> MPQLHYVPYDTPVEDVMRILKESGTLVIRNFLDQNTVQKVQDEVDDYVRNWNPGPGSKTKQPSNLSLMSKTYRCEVLNHPWMHAICERMFGPTYGDYWFNGGSILHLEPGENTQPIHQDHVFYQISKWRRPTDPDLTINFTMALTEFTVENGGTRVCPGSHLWENGHASPAEEDMVPVLMQPGDALILPGSMWHSAGANRTSEYRRGFATSFHPCHFTPIESHHHLPREMVEEMTPLVQKMLGFRTLNLHNNVKVWKAGEGNLEDATGLKSVAAKLAAALEHHHHHH

Here, we report the biochemical and structural characterizations of the unusually promiscuous and catalytically versatile Fe/αKG oxygenase SptF, involved in the biosynthesis of fungal meroterpenoid emervaridones. The in vitro analysis revealed that SptF catalyzes several continuous oxidation reactions, including hydroxylation, desaturation, epoxidation, and skeletal rearrangement. Fe/αKG oxygenases utilize αKG as a co-substrate and Fe(II) as a cofactor. Through the oxidative decarboxylation of αKG, a reactive Fe(IV)-oxo intermediate is generated to activate a selective aliphatic C–H bond, which is normally difficult to cleave due to high bond-dissociation energy, and then oxidative products are generated following radical recombination.

To further investigate the importance of the flexible lid-like loop region, with a length of 19 amino acid residues, we tested truncated loops. Based on the sequence comparison as well as the structures of SptF in complex with 1, loop-truncated variants of 6 residues (His61-Val66), 9 residues (Lys58-Val66), 16 residues (Asn54-Lys69), and 19 residues (Trp53-Lys71) were constructed. Since the Δ19 variant was expressed in inclusion bodies, the Δ6, Δ9, and Δ16 variants were tested for their enzyme reaction activities with 1, 2, and 3. Interestingly, although the activities of the truncated variants were dramatically decreased as compared to the wild-type, all the loop-truncated variants still consumed 60–94% and 17–77% of 1 and 2 over 24 h, respectively, and generated many minor products, including the E-ring-opened product 32, but not 3–5. On the other hand, these variants also showed 26–56% activities toward 3 and generated small amounts of 4 and 5, as well as other minor compounds. Although we could not determine the structures of the minor products due to low yields, these results suggested that the lid-like region is not essential for the reactions with 1–3, but important for the reaction efficiency and product selectivity. We also tested the activities of the truncated variants with unnatural substrates, including the fungal meroterpenoids 10 and 13, and steroids 21, 24, and 28. As a result, all the variants still maintained 24–40% and 56–84% activities toward 10 and 13, but dramatically decreased activities toward 21, 24, and 28 (<20%). The kinetics analysis of the loop-truncation variant Δ9 revealed that the variants also maintained comparable activity toward 15 to that of wild-type. Thus, the mutagenesis and kinetic assay results strongly suggest that the malleability of the lid-like loop region contributes to the remarkable substrate promiscuity and catalytic versatility of SptF.> MVVLDKKLLERLTSRKVPLEELEDMEKRCFLSTFTYQDAFDLGTYIRNAVKENFPEKPVAIDISLPNGHCLFRTVTYGGSALDNDFWIQRKKKTALRFGHSSFYMGCKKGDKTPEEKFFVDSKEYAFHGGAVLIQSERSDYPYACLTISGLKQEEDHLMALSSLIAFANESLEEDLNLD;> MVVLDKKLLERLTSRKVPLEELEDMEKKCFLSTFTYQDAFDLGTYIKNAVKENFPDKPVAIDISLPNGHCLFRTVTYGGSALDNDFWIQRKKKTALRFGHSSFYMGCKKGDKTPEEKFFVDSKEYAFHGGAVLIQSERSTYPYACLTISGLKQEEDHLMAVS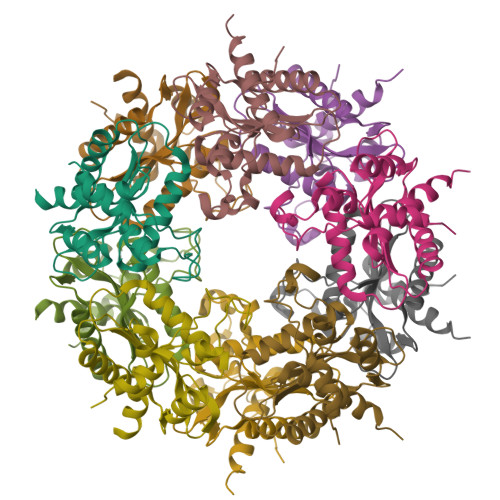SLIAFANESLEEDLNLD;> MVVLDKKLLERLTSRKVPLEELEDMEKRCFLSTFTYQDAFDLGTYIRNAVKENFPEKPVAIDISLPNGHCLFRTVTYGGSALDNDFWIQRKKKTALRFGHSSFYMGCKKGDKTPEEKFFVDSKEYAFHGGAVLIQSERSDYPYACLTISGLKQEEDHLMAVSSLIAFANESLEEDLNLD;> MVVLDKKLLERLTSRKVPLEQLEDMEKRCFLSTFTYQDAFDLGTYIRNAVKENFPEKPVAIDISLPNGHCLFRTVTYGGSALDNDFWIQRKKKTALRFGHSSFYMGCKKGDKTPEEKFFVDSKEYAFHGGAVLIQSERSDYPYACLTISGLKQEEDHLMAVSSLIAFANESLEEDLNLD;> MVVLDKKLLERLTSRKTPLEELEDMEKRCFLSTFTYQDAFDLGTYIRNAVKENFPEKPVAIDISLPNGHCLFRTVTYGGSALDNDFWIQRKKKTALRFGHSSFYMGCKKGDKTPEEKFFVDSKEYAFHGGAVLIQSERSDYPYACLTISGLKQEEDHLMAVSSLIAFANESLEEDLNLD> SLTGEPAPVLSSPPPADVSTFLAFPSPEKLLRLGPKSSVLIAQQTDTSDPEKVVSAFLKVSSVFKDEATVRMAVQDAVDALMQKAFNSSSFNSNTFLTRLLVHMGLLKSEDKVKAIANLYGPLMALNHMVQQDYFPKALAPLLL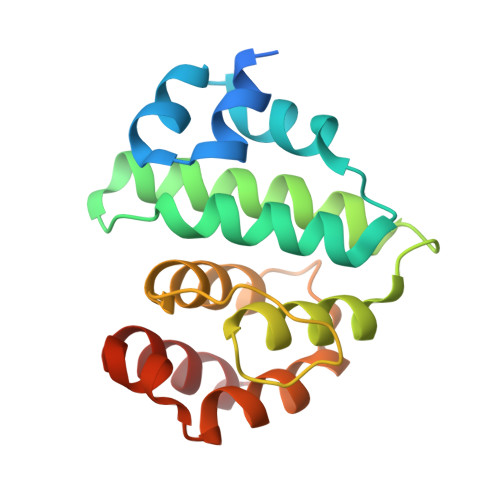AFVTKPNSALESCSFARHSLLQTLYKV>MVGYSSKLIFVSMITRHGDRAPFANIENANYSWGTELSELTPIGMNQEYNLGLQLRKRYIDKFGLLPEHYVDQSIYVLSSHTNRTVVSAQSLLMGLYPAGTGPLIGDGDPAIKDRFQPIPIMTLSADSRLIQFPYEQYLAVLKKYVYNSPEWQNKTKEAAPNFAKWQQILGNRISGLNDVITVGDVLIVAQAHGKPLPKGLSQEDADQIIALTDWGLAQQFKSQKVSYIMGGKLTNRMIEDLNNAV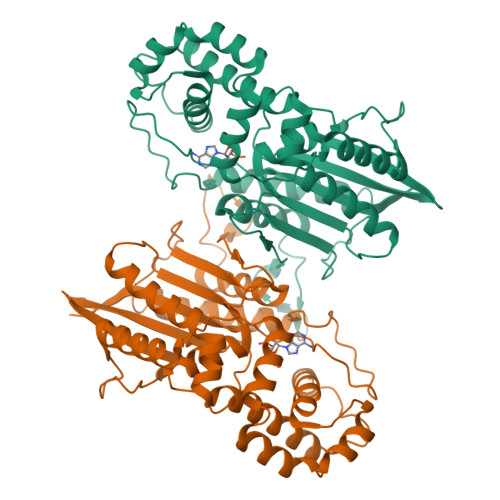NGKSKYKMTYYSGHALTLLEVMGTLGVPLDTAPGYASNLEMELYKDGDIYTVKLRYNGKYVKLPIMDKNNSCSLDALNKYMQSINEKFQKHHHHHH[2x]> MESKRNKPG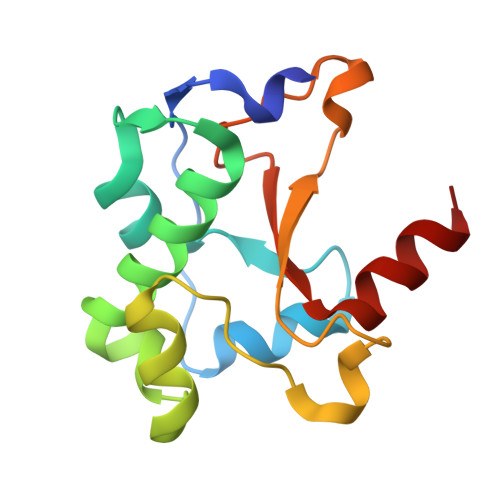KATGKGKPVGDKWLDDAGKDSGAPIPDRIADKLRDKEFKSFDDFRKAVWEEVSKDPELSKNLNPSNKSSVSKGYSPFTPKNQQVGGRAVYELHHDKPISQGGEVYDMDNIRVTTPKRHIDIHRGK>HGGEAHMVPMDKTLKEFGADVQWDDYAQLFTLIKDGAYVKVKPGAQTAIVNGQPLALQVPVVMKDNKAWVSDTFINDVFQSGLDQTFQVEKRPHPLNALTADEIKQAVEIVKASADFKPNTRFTEISLLPPDKEAVWAFALENKPVDQPRKADVIMLDGKHIIEAVVDLQNNKLLSWQPIKDAHGMVLLDDFASVQNIINNSEEFAAAVKKRGITDAKKVITTPLTVGYFDGKDGLKQDARLLKVISYLDVGDGNYWAHPIENLVAVVDLEQKKIVKIEEGPVVPVPMTARPFDGRDRVAPAVKPMQIIEPEGKNYTITGDMIHWRNWDFHLSMNSRVGPMISTVTYNDNGTKRKVMYEGSLGGMIVPFGDPDIGWYFKAYLDSGDYGMGTLTSPIARGKDAPSNAVLLNETIADYTGVPMEIPRAIAVFERYAGPEYKHQEMGQPNVSTERRELVVRWISTVGNYDYIFDWIFHENGTIGIDAGATGIEAVKGVKAKTMHDETAKDDTRYGTLIDHNIVGTTHQHIYNFRLDLDVDGENNSLVAMDPVVKPNTAGGPRTSTMQVNQYNIGNEQDAAQKFDPGTIRLLSNPNKENRMGNPVSYQIIPYAGGTHPVAKGAQFAPDEWIYHRLSFMDKQLWVTRYHPGERFPEGKYPNRSTHDTGLGQYSKDNESLDNTDAVVWMTTGTTHVARAEEWPIMP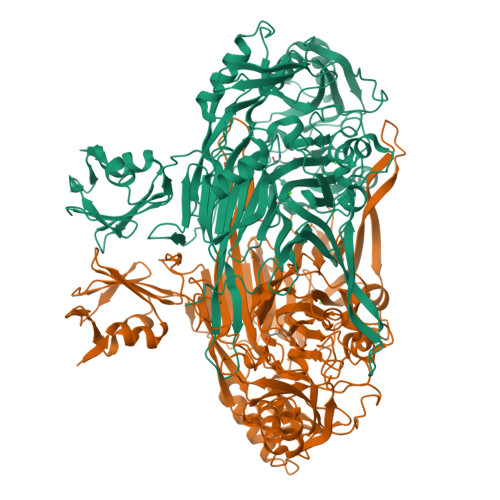TEWVHTLLKPWNFFDETPTLGALKKDK[2x]>[14x]MHRTYSLRNSRAPTASQLQNPPPPPSTTKGRFFGKGGLAYSFRRSAAGAFGPELSRKLSQLVKIEKNVLRSMELTANERRDAAKQLSIWGLENDDDVSDITDKLGVLIYEVSELDDQFIDRYDQYRLTLKSIRDIEGSVQPSRDRKDKITDKIAYLKYKDPQSPKIEVLEQELVRAEAESLVAEAQLSNITRSKLRAAFNYQFDSIIEHSEKIALIAGYGKALLELLDDSPVTPGETRPAYDGYEASKQIIIDAESALNEWTLDSAQVKPTLSFKQDYEDFEPEEGEEEEEEDGQGRWSEDEQEDGQIEEPEQEEEGAVEEHEQVGHQQSESLPQQTTA

The yeast eisosome, composed of the BAR-domain proteins Pil1 and Lsp1 (hereafter, Pil1/Lsp1), scaffolds a membrane compartment that senses and responds to mechanical stress by flattening and releasing sequestered factors. MCC–eisosomes are relatively stable, and have been implicated in sensing and responding to plasma membrane stress: various stimuli, including hypo-osmotic shock, heat shock and mechanical pressure, cause eisosomes to flatten and release sequestered proteins to affect signalling or transport functions. Here we isolated near-native eisosomes as helical tubules made up of a lattice of Pil1/Lsp1 bound to plasma membrane lipids, and solved their structures by helical reconstruction.

Our final reconstructions were made with three lipid mixtures: (1) ‘minus PI(4,5)P2/plus sterol’ (‘−PI(4,5)P2/+sterol’), containing 30% cholesterol; (2) ‘plus PI(4,5)P2/minus sterol’ (‘+PI(4,5)P2/−sterol’), containing 10% PI(4,5)P2; and (3) ‘plus PI(4,5)P2/plus sterol’ (‘+PI(4,5)P2/+sterol’), containing 10% PI(4,5)P2 and 15% cholesterol. For all three lipid mixtures, the overall architecture of the Pil1 lattice is similar to the native-source samples. In the +PI(4,5)P2/−sterol samples, the AH density is improved, and the AH density resolution is best and most resembles that of the native-source eisosomes in the +PI(4,5)P2/+sterol samples, which suggests that PI(4,5)P2 is crucial for AH stabilization. One feature that was notably absent from the +PI(4,5)P2/−sterol helices was the pattern of membrane voids in the cytoplasmic leaflet that we observe in the native-source eisosome filaments. Notably, these conserved residues were previously shown to be important for eisosome assembly in vivo and membrane binding in vitro. This extra density, not present in the −PI(4,5)P2/+sterol Pil1 filaments, is likely to reflect a PI(4,5)P2-binding site in the native-source eisosomes. In addition, in the CG MD simulations for both the +PI(4,5)P2/−sterol and the +PI(4,5)P2/+sterol systems, PI(4,5)P2 occupancy was increased at charged residues in the lipid-binding pocket, especially residues R43, Q60, R126, K130 and R133.>SNAMHRSRVSTVLIDVPREQASRSAQFWAGALGVRADSPPGEPQYVTLHGALPGLVTAVQALEEGEARYHL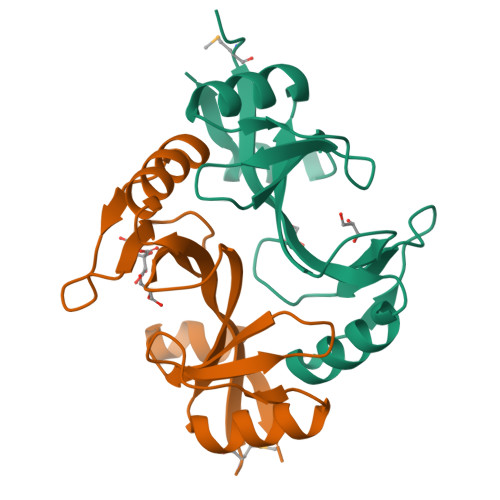DIETDDVDAEVERLVGLGAVEESSWQGCRTLRVPGGQLVCVIPLHSDPDEFAARATSWP[2x]> MSNKEKNASETRKAYTTKMIPRSHDRMKLLGNFMDYLMDGTPIFFELWNQFGGGIDRDIISGTANKDKISDDLLLAVNWFKVMPINSKPQGVSPSNLANLFQQYSGSEPDIQAQEYFASNFDTEKHQWKDMRVEYERLLAELQLSRSDMHHDLKLMYKEKCIGLSLSTAHYITSVMFGTGAKNNRQTKHQFYSKVIQLLEESTQINSVEQLASIILKAGDCDSYRKLRIRCSRKGATPSILKIVQDYELGTNHDDEVNVPSLIANLKEKLGRFEYECEWKCMEKIKAFLASKVGPYYLGSYSAMLENALSPIKGMTTKNCKFVLKQIDAKNDIKYENEPFGKIVEGFFDSPYFESDTNVKWVLHPHHIGESNIKTLWEDLNAIHSKYEEDIASLSEDKKEKRIKVYQGDVCQTINTYCEEVGKEAKTPLVQLLRYLYSRKDDIAVDKIIDGITFLSKKHKVEKQKINPVIQKYPSFNFGNNSKLLGKIISPKDKLKHNLKCNRNQVDNYIWIEIKVLNTKTMRWEKHHYALSSTRFLEEVYYPATSENPPDALAARFRTKTNGYEGKPALSAEQIEQIRSAPVGLRKVKKRQMRLEAARQQNLLPRYTWGKDFNINICKRGNNFEVTLATKVKKKKEKNYKVVLGYAANIVRKNTYAAIEAHANGDGVIDYNDLPVKPIESGFVTVESQVRDKSYDQLSYNGVKLLYCKPHVESRRSFLEKYRNGTMKDNRGNNIQIDFMKDFEAIADDETSLYYFNMKYCKLLQSSIRNHSSQAKEYREEIFELLRDGKLSVLKLSSLSNLSFVMFKVAKSLIGTYFGHLLKKPKNSKSDVKAPPITDEDKQKADPEMFALRLALEEKRLNKVKSKKEVIANKIVAKALELRDKYGPVLIKGENISDTTKKGKKSSTNSFLMDWLARGVANKVKEMVMMHQGLEFVEVNPNFTSHQDPFVHKNPENTFRARYSRCTPSELTEKNRKEILSFLSDKPSKRPTNAYYNEGAMAFLATYGLKKNDVLGVSLEKFKQIMANILHQRSEDQLLFPSRGGMFYLATYKLDADATSVNWNGKQFWVCNADLVAAYNVGLVDIQKDFKKKLEHHHHHH

Cas12i is a newly identified member of the functionally diverse type V CRISPR-Cas effectors. Among them, Cas12i is characterized by a relatively smaller size (1033-1093aa) compared with Cas12a. Cas12i has substantially different efficiencies in cutting two strands of target DNA, which results in a nicking activity that could be utilized to develop a double-nicking approach for genome editing with high specificity. In Cas12i1, the REC lobe consists of the Helical-I domain and the PAM-interacting (PI) domain, whereas the NUC lobe comprises the Wedge (WED), Helical-II, RuvC, and Nuc domains.

To obtain these crystal structures, the crystal structure of the selenomethionine (SeMet)-labeled wild-type Cas12i1 ternary complex was solved using the single-wavelength anomalous diffraction method. Next, the SeMet-labeled model was used to solve the crystal structures of two unlabeled ternary complexes using the molecular replacement method. In the pre-cleavage R-loop complex, the two strands of target DNA are unwound beyond the PAM duplex and the TD strand forms a 19-bp heteroduplex with the crRNA guide region. The NTD strand extends from the PAM duplex and is partially exposed to the surrounding solvent. The nucleotides dT(4*)–dA(6*) of the NTD strand are disordered and invisible due to the flexibility, and the nucleotides dA(7*)–dG(20*) pass through the channel formed by the Helical-I, Helical-II, RuvC, and Nuc domains. The structure of the pre-cleavage R-loop complex displays how the NTD strand is accommodated within the RuvC active site. Side chains of three catalytic residues D647 (virtual modeling of A647D), E894, and D1074 in the RuvC domain point toward the phosphate group between the nucleotides dG(15*) and dC(16*), implying this position as the possible cutting site in the NTD strand.>MDPPVTHDLRVSLEEIYSGCTKKMKISHKRLNPDGKSIRNEDKILTIEVKKGWKEGTKITFPKEGDQTSNNIPADIVFVLKDKPHNIFKRDGSDVIYPARISLREALCGCTVNVPTLDGRTIPVVFKDVIRPGMRRKVPGEGLPLPKTPEKRGDLIIEFEVIFPERIPQTS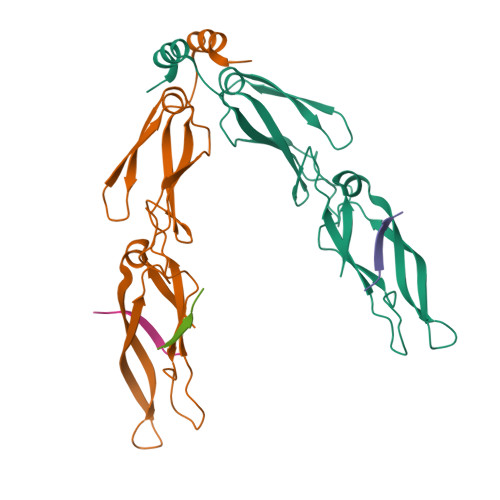RTVLEQVLPI[2x];>GPTIEEVD[3x]> MTRDQNGTWEMESNENFEGYMKAL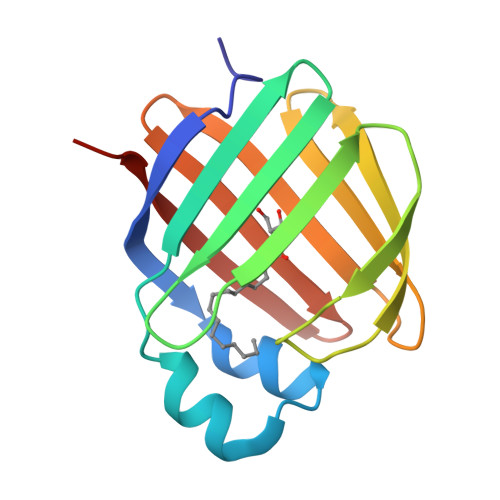DIDFATRKIAVRLTQTKVIDQDGDNFKTKTTSTFRNYDVDFTVGVEFDEYTKSLDNRHVKALVTWEGDVLVCVQKGEKENRGWKQWIEGDKLYLELTCGDQVCRQVFKKKLVPR> MSQVTDMRSNSQGLSLTDSVYERLLSERIIFLGSEVNDEIANRLCAQILLLAAEDASKDISLYINSPGGSISAGMAIYDTMVLAPC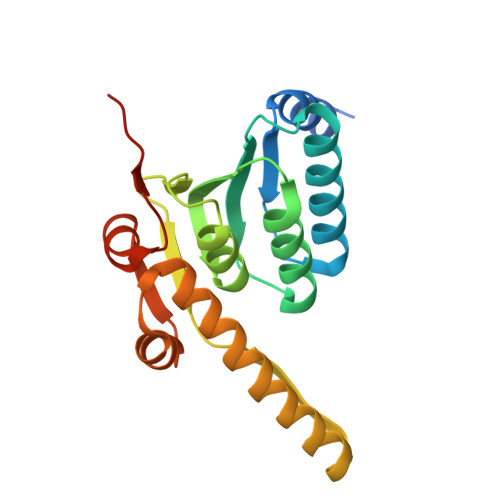DIATYAMGMAASMGEFLLAAGTKGKRYALPHARILMHQPLGGVTGSAADIAIQAEQFAVIKKEMFRLNAEFTGQPIERIEADSDRDRWFTAAEALEYGFVDHIITRAHVNGEAQ>ASNAMHEWGLSEELKIQTKQMIEIAEKELSIMRNAIDKEDECILCKMEDIHHMLANVQTLAATYYIQAYLSPYTESSSFITTAIQHLSARKHGALIVVERNETLEALIQTGTTLNAHLTAPLLESIFYPGNPLHDGAVLVKNNHIVSAANILPLTKST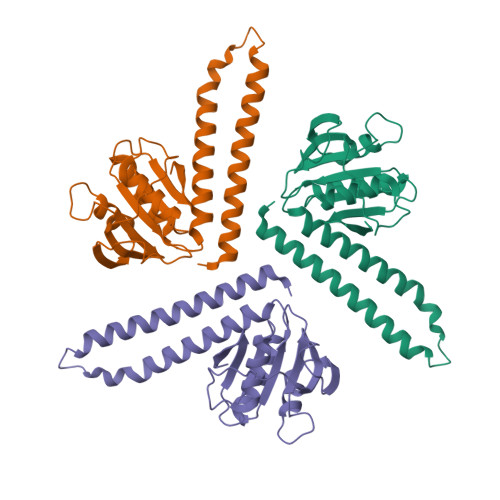EVDPELGTRHRAAIGLSEKSDALILVVSEETGRTSFALNGILYTISL[3x]> GSMKLPTNLAYERSIDPSDVCFFVVWPDDRKTPLTYNSRTLLGQMEAASLAYDVSGQPIKSATAEALAQGNPHQVDFCHVPYGASHIECSFSVSFSSELRQPYKCNSSKVKQTLVQLVELYETKIGWTELATRYLMNICNGKWLWKNTRKAYCWNIVLTPWPWNGEKVGFEDIRTNYTSRQDFKNNKNWSAIVEMIKTAFSSTDGLAIFEVRATLHLPTNAMVRPSQVFTEKESGSKSKS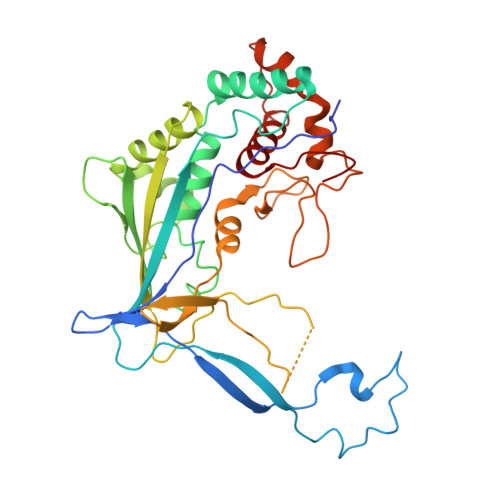KTQNSRVFQSTTIDGERSPILGAFKTGAAIATIDDWYPEATEPLRVGRFGVHREDVTCYRHPSTGKDFFSILQQAEHYIEVLSANKTPAQETINDMHFLMANLIKGGMFQHKGD> EV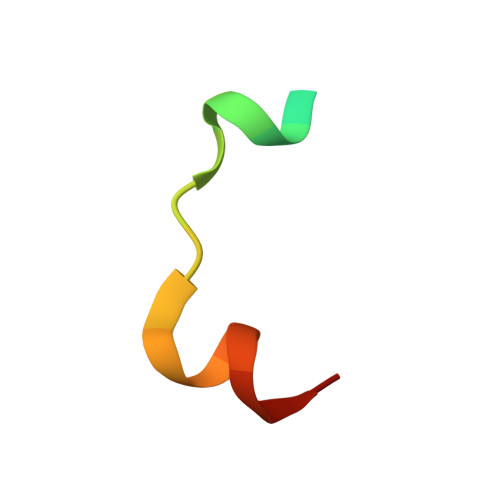KPKNKARRRTTTQMELLYAD> QGLYVGGFVDVVSCPKLEQELYLDPDQVTDYLPVTEPLPI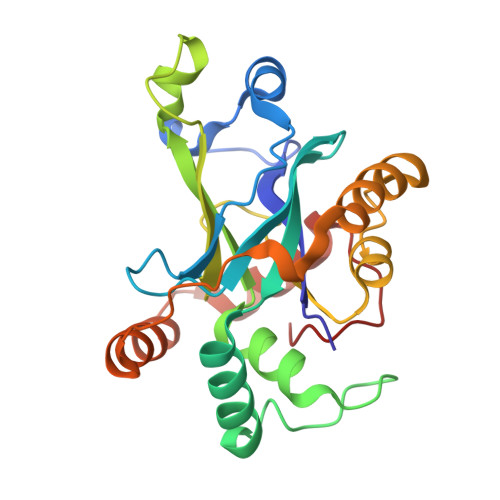TIEHLPETEVGWTLGLFQVSHGIFCTGAITSPAFLELASRLADTSHVARAPVKNLPKEPLLEILHTWLPGLSLSSIHPRELSQTPSGPVFQHVSLCALGRRRGTVAVYGHDAEWVVSRFSSVSKSERAHILQHVSSCRLEDLSTPNFVSPLETLMAKAIDAGFIRDRLDLLKTDRGVASILSPVYLKA> SDTVDIYDDRGKLLESNVDIMSLAPTRNAAIQSIIMDTKRSVAVNLAGIQGALASGKMGGKGRQILGRGLNYDIVGNADAIAENVKKLVQVDEGDDTNVIKVKGGKSLLIQSPKSRIIAGADFMSATTVGAAAVTQTIMDMFGTDPYDAPIVKSAVWGSYPQTMDLMGGQVQGILSIPQNNEGLGFSLRNIMANHVAAISNRNAMNASALSSIYEQSGIFEMGGAVGMFERHQLLGLAYQGLNANNLLYDIVKENGKDGTIGTVIESVVRRAIEAGIISVDKTAPSGYNFYKANDVPKWNACAAVGTLAATLVNCGAGRAAQNVSSTLLYFNDILEKETGLPGCDYGKVEGTAVGFSFFSHSIYGGGGPGVFNGNHVVTRHSRGFAIPCVCAAVALDA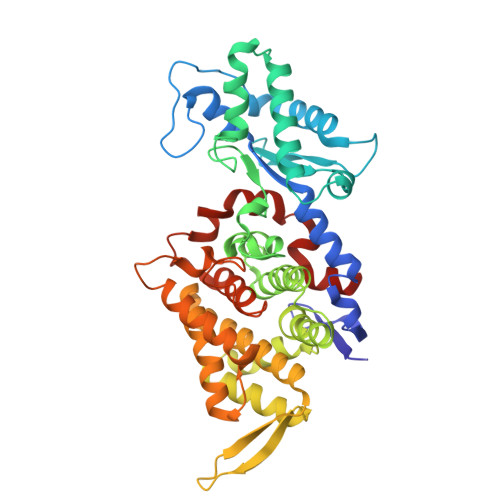GTQMFSIESTSGLIGDVFGAIPEFREPIKAVAGVL4-ethylphenol | C8 H10 O | 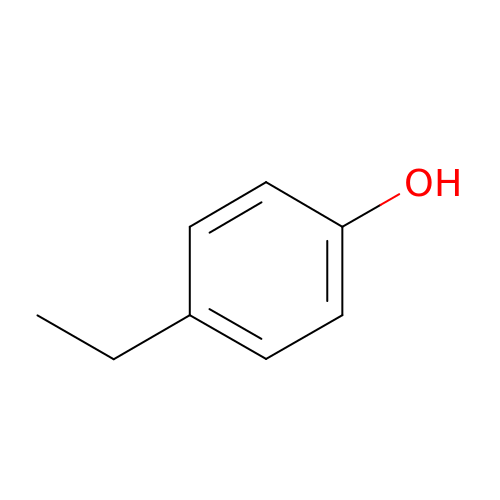HXDOZKJGKXYMEW-UHFFFAOYSA-N>PSVYDAAAQLTADVKKDLRDSWKVIGSDKKGNGVALMTTLFADNQETIGY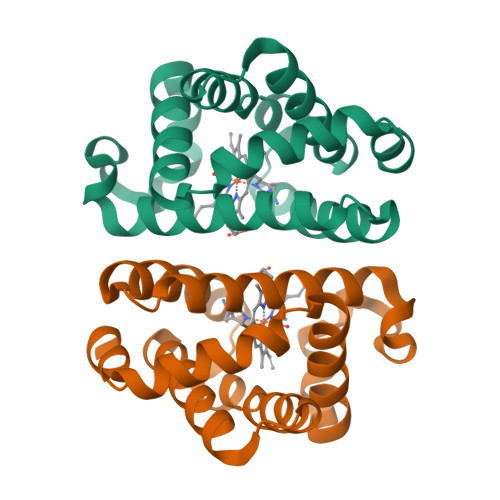FKRLGDVSQGMANDKLRGVSITLMYALQNFIDQLDNPDDLVCVVEKFAVNHITRKISAAEFGKMNGPIKKVLASKNFGDKYANAWAKLVAVVQAAL[2x]> GASVDAFKILEDPKWEFPRKNLVLGKTLGEGEFGKVVKATAFHLKGRAGYTTVAVKMLKENASPSELRDLLSEFNVLKQVNHPHVIKLYGACSQDGPLLLIVEYAKYGSLRGFLRESRKVGPGYLGSGGSRNSSSLDHPDERALTMGDLISFAWQISQGMQYLAEMKLVHRDLAARNILVAE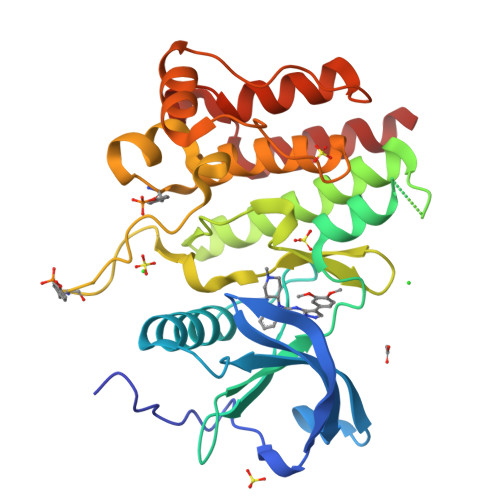GRKMKISDFGLSRDVYEEDSYVKRSQGRIPVKWMAIESLFDHIYTTQSDVWSFGVLLWEIVTLGGNPYPGIPPERLFNLLKTGHRMERPDNCSEEMYRLMLQCWKQEPDKRPVFADISKDLEKMMVKRR>LDGPYQPTNFKPPNDYWILLNPTNQQVVLEGTNKTDIWVALLLVEPNVTNQSRQYTLFGETKQITVENNTNKWKFFEMFRSNVSAEFQHKRTLTSDTKLAGFMKFYNSVWTFHGETPHATTDYSSTSNLSEVETVIHVEFYIIPRSQESKCSEYINTGL[4x]

The protease-sensitive VP4 proteins protrude from the outer capsid shell, forming sixty spikes that are responsible for host receptor interactions. Each VP4 protein is cleaved by trypsin into two domains, VP5* and VP8*, corresponding to the stalk and the distal head of the spike protein, respectively. The distal VP8* head interacts with RV host glycan receptors for viral attachment, while the VP5* stalk assists in viral penetration into host cells. The RV VP8* domain adopts a classical galectin-like fold with the central structure being an anti-parallel β-sandwich formed by a five-stranded β-sheet and a six-stranded β-sheet.

The crystal structures of P (strain BM11596) and P (strain BM11596) in complex with LNFP I were solved. The VP8* of P BM11596 strain adopted a classical galectin-like fold as similar to other known VP8* structures, with two twisted antiparallel β-sheets consisting of strands A, L, C, D, G, H and M, B, I, J, K, respectively. The specific interactions between LNFP I and P VP8* were revealed by the crystal structure. The Galβ1-3GlcNAc type 1 precursor in the LNFP I-bound P VP8* inserted into the pocket formed by W81, M167, A183, T184, T185, R209, E212, and appeared to be stabilized through hydrogen bonding and hydrophobic interactions. The Gal-IV moiety was stabilized by F168, Y170, and W174 through hydrophobic interactions and the terminal Glc-V moiety was stabilized by Y170, S172, Y187 though hydrophobic interactions and N171 through hydrogen bonding. The Fuc-I pointed away from the protein surface, consistent with the STD NMR results. Some key residues involved in the binding pocket in the P[II] genogroup are highly conserved, e.g. W81 in the βB strand, W174 in the βJ strand, T184 and T185 in the βK strand, R209 in the βm-αA loop, and E212 in the αA helix. These highly conserved key residues in the P[II] genogroup are consistent with the crystal structures showing that P /P /P /P in the P[II] genotype can bind the Lewis negative type 1 HBGAs in the βα site. From the recent X-ray crystallography studies, it was found that P, P, P, P employed the βα binding site to accommodate H type 1 ligand LNFP I, which is consistent with our NMR-driven HADDOCK results.> AGMSLTQVSGPVYVVEDNYYVQENSMVYFGAKGVTVVGATWTPDTARELHKLIKRVSRKPVLEVINTNYHTDRAGGNAYWK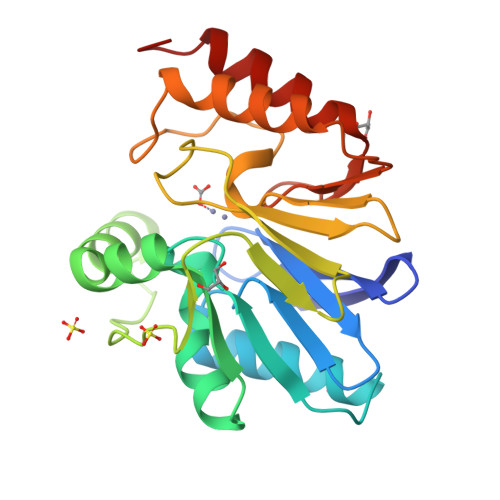SIGAKVVSTRQTRDLMKSDWAEIVAFTRKGLPEYPDLPLVLPNVVHDGDFTLQEGKVRAFYAGPAHTPDGIFVYFPDEQVLYGGCILKEKLGNLSFADVKAYPQTLERLKAMKLPIKTVIGGHDSPLHGPELIDHYEALIKAAPQSS>[2x]LTFESTSRFAEVDVDGPLKLHYHEAGVGNDQTVVLLHGGGPGAASWTNFSRNIAV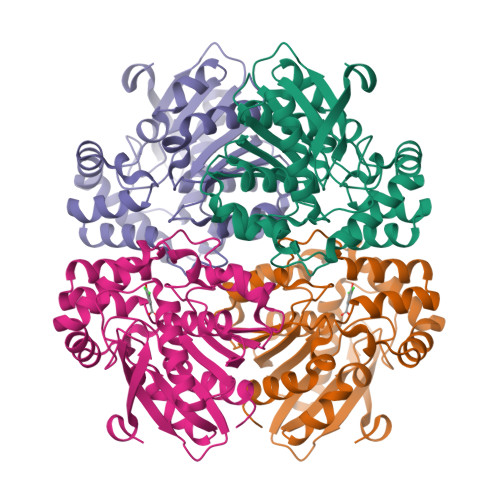LARHFHVLAVDQPGYGHSDKRAEHGQFNRYAAMALKGLFDQLGLGRVPLVGNSLGGGTAVRFALDYPARAGRLVLMGPGGLSINLFAPDPTEGVKRLSKFSVAPTRENLEAFLRVMVYDKNLITPELVDQRFALASTPESLTATRAMGKSFAGADFEAGMMWREVYRLRQPVLLIWGREDRVNPLDGALVALKTIPRAQLHVFGQCGHWVQVEKFDEFNKLTIEFLGGG> MVRPVVG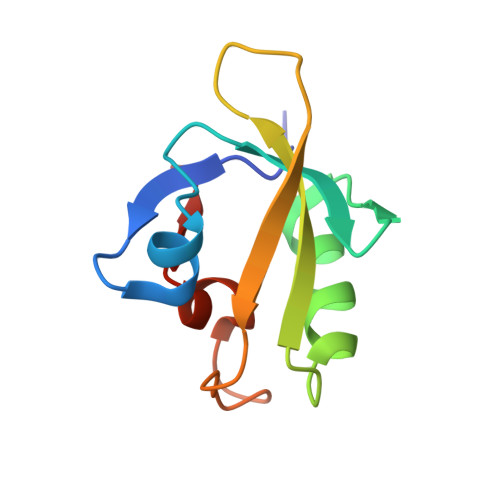EIAANSIAAEAQIAPGTELKAVDGIETPDWDAVRLQLVDKIGDESTTITVAPFGSDQRRDVKLDLRHWAFEPDKEDPVSSLGIRPRGP>SPPAVPQTFQVAHLHAPTGSGKSTKVPAAYAAQGYKVLVLNPSVAATLGFGAYMSKAHGIDPNIRTGVRTITTGAPITYSTYGKFLADGGCSGGAYDIIICDECHSTDSTTILGIGTVLDQAETAGARLVVLATATPPGSVTVPHPNIEEVALSSTGEIPFYGKAIPIETIKGGRHLI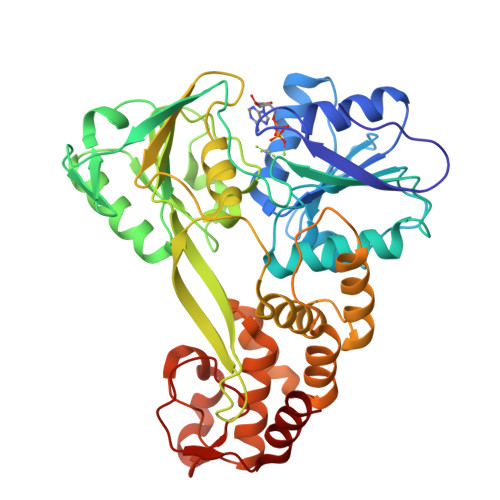FCHSKKKCDELAAKLSGLGLNAVAYYRGLDVSVIPTSGDVIVVATDALMTGFTGDFDSVIDCNTCVTQTVDFSLDPTFTIETTTVPQDAVSRSQRRGRTGRGRMGIYRFVTPGERPSGMFDSSVLCECYDAGCAWYELTPAETSVRLRAYLNTPGLPVCQDHLEFWESVFTGLTHIDAHFLSQTKQAGDNFPYLVAYQATVCARAQAPPPSWDQMWKCLIRLKPTLHGPTPLLYRLGAVQNEVTTTHPITKYIMACMSA[2x]> MGSMISTPEPLHAGHILTPFCCGVDSIDNWLKQRAMKNQTTGASRTFVCCGSDSNVLAYYSLASSAVTTNTSPGRFRRNMPDPIPVVVLGRLAVDKSLHGQGVARALVRDAGLRVIQVAETIGIRGMLVHALSDEAREFFQRVGFV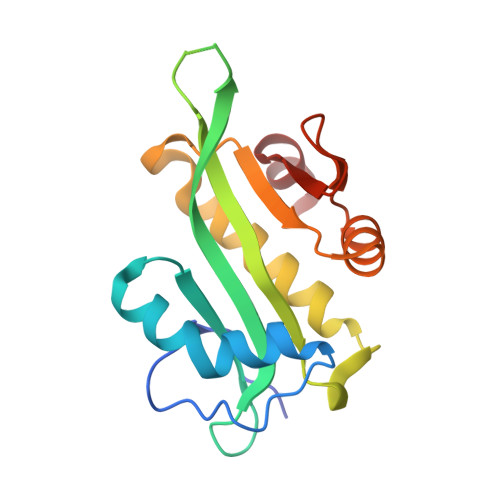PSPMDPMMLMVTLGDLVESV Phylogenetically diverse bacteria can carry out chloramphenicol reduction, but only a single enzyme has been described that efficiently catalyzes this reaction, the NfsB nitroreductase from Haemophilus influenzae strain KW20. We found that expression of H. influenzae and Neisseria spp. nfsB genes, but not Pasteurella multocida nfsB, allows Escherichia coli to resist chloramphenicol by nitroreduction. Mass spectrometric analysis confirmed that purified H. influenzae and N. meningitides NfsB enzymes reduce chloramphenicol to amino-chloramphenicol, while kinetics analyses supported the hypothesis that chloramphenicol reduction is a secondary activity. Previous kinetic studies of nitroreductase catalysis revealed that reactions progress by a double-displacement (ping-pong) mechanism that appears to lack the gating steps necessary to impose specificity, explaining the substrate promiscuity of these enzymes.

To understand better how variation in the substrate-binding site mediates activity, we solved the crystal structures of the NfsB homologs from Hi KW20, Hi Int1, Hi 86-028NP, and Nm Z2491. The Hi Int1 and Hi 86-028NP enzymes showed comparable, although statistically significant, kinetics (q < 0.05) to Hi KW20 NfsB. In contrast to the reduction of chloramphenicol, the oxidation of NADPH showed less apparent variability in catalytic efficiency, with only Hi 86-028NP NfsB showing significantly greater activity than Hi KW20 NfsB (∼1.7-fold, q < 0.005). The relative increase in resistance conferred by H. influenzae or Neisseria nfsB expression ranged from approximately a 16-fold increase (Hi KW20 and Hi 86-028NP) down to an ∼2-fold increase (Hi Int1 and Hi 12). Intuitively, the Ser68-Met74 pair found in Hi 12 NfsB would provide more of the flexibility needed to properly locate and orient Trp71 to make space for the ribose of NADP than the Pro68-Ile74 pair in other H. influenzae NfsB homologs (Pro68-Ala74 in Nm Z2491 NfsB).

>SNAMTQLTREQVLELFHQRSSTRYYDPAKKISDEDFECILECGRLSPSSVGSEPWKFLVIQNKTLREKMKPFSWGMINQLDNCSHLVVILAKKNARYDSPFFVDVMARKGLNAEQQQAALAKYKALQEEDMKLLENDRTLFDWCSKQTYIALANMLTGASALGIDSCPIEGFHYDKMNECLAEEGLFDPQEYAVSVAATFGYRSRDIAKKSRKGLDEVVRWVG[4x]> MSDITKIKQEFDKKVAEIQALMKNPQQDSGLLSNSIDFRDQNLIFSNSGGVCTSSKDKIENYPAKGYPYKRGVKLSFGDGTTELEVEAGGGDDLYGVCSDIDEFSGMATVIPITNNFTGYLTLKKDGQNGVNPGDKLNFNQHG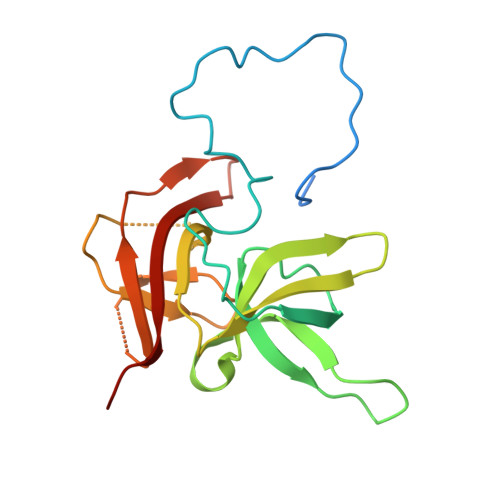ELEKVTGAQKSVNAIALSKAHKLTEDLFIVLASVFGNRAIKG> KETAAAKFERQHMDSSTSAASSSNYCNQMMKSRNLTKDRCKPVNTFVHESLADVQAVCSQKNVACKNGQTNCYQSYSTMSITDCRET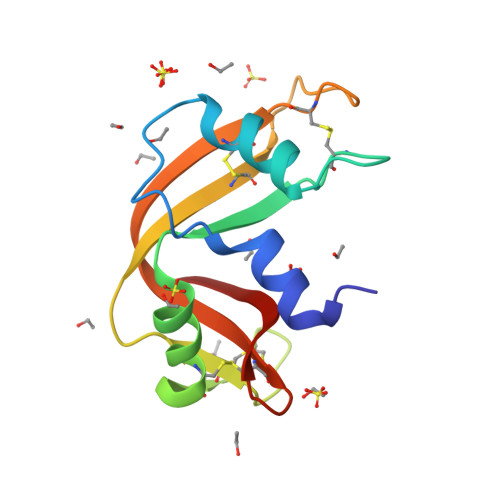GSSKYPNCAYKTTQANKHIIVACEGNPYVPVHFDASV[2,4-bis(oxidanyl)phenyl]-phenyl-methanone 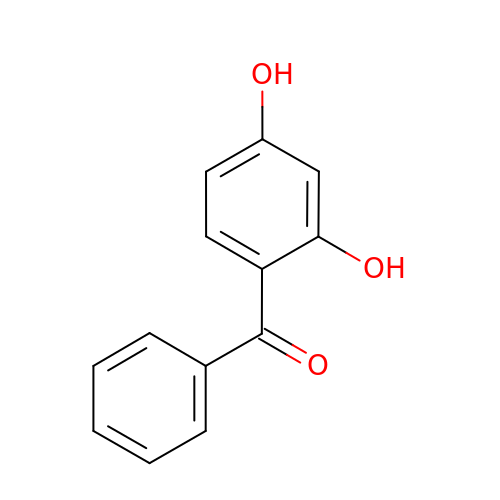| C13 H10 O3 | ZXDDPOHVAMWLBH-UHFFFAOYSA-N>[3x]MAYSQGGGKKKVCYYYDGDIGNYYYGQGHPMKPHRIRMTHNLLLNYGLYRKMEIYRPHKAT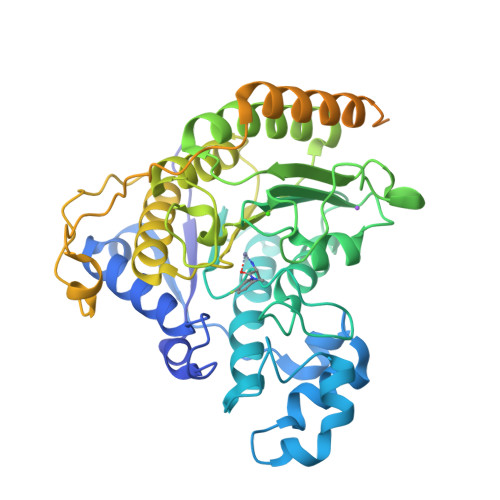AEEMTKYHSDEYIKFLRSIRPDNMSEYSKQMQRFNVGEDCPVFDGLFEFCQLSTGGSVAGAVKLNRQQTDMAVNWAGGLHHAKKSEASGFCYVNDIVLAILELLKYHQRVLYIDIDIHHGDGVEEAFYTTDRVMTVSFHKYGEYFPGTGDLRDIGAGKGKYYAVNFPMRDGIDDESYGQIFKPIISKVMEMYQPSAVVLQCGADSLSGDRLGCFNLTVKGHAKCVEVVKTFNLPLLMLGGGGYTIRNVARCWTYETAVALDCEIPNELPYNDYFEYFGPDFKLHISPSNMTNQNTPEYMEKIKQRLFENLRMLPHAPGVQMQAIPEDAVHEDSGDEDGEDPDKRISIRASDKRIACDEEFSDSEDEGEGGRRNVADHKKGAKKARIEEDKKETEDKKTDVKEEDKSKDNSGEKTDTKGTKSEQLSNPGSSGHHHHHH>MGSSHHHHHHSSGRENLYFQGMDYFRLAEKFLREMHAKYMKRVSRPGNTPRPWFDFSEERLLSRLFEEMDEL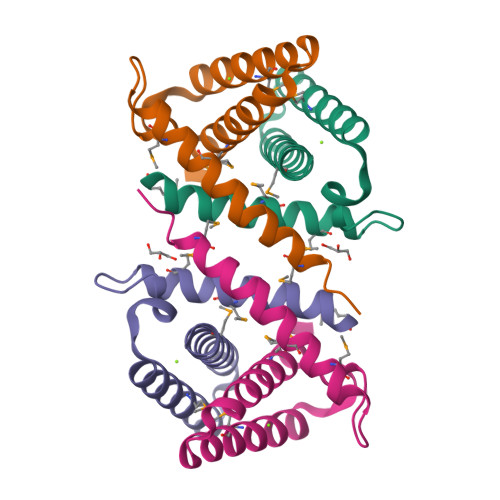REAVEKEDWENLRDELLDVANFCMYLWGKLSVKNIYDKGEEQ[2x]> GSMTDGDYDYLIKLLALGDSGVGKTTFLYRYTDNKFNPKFITTVGIDFREKRVVYDTQGADGASGKAFKVHLQLWDTAGLERFRSLTTAFFRDAMGFLLMFDLTSQQSFLNVRNWMSQLQANAYCENPDIVLIGNKADLPDQREVNERQARELAEKYGIPYFETSAATGQ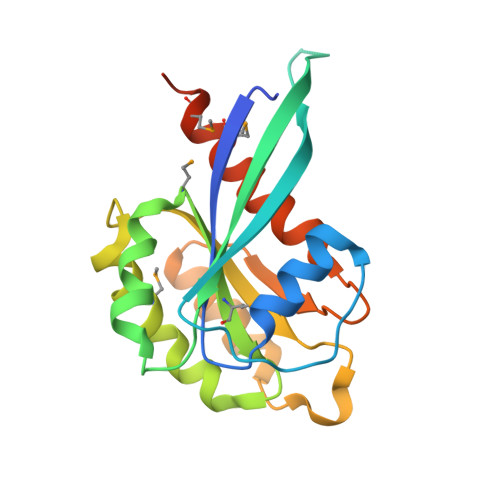NVEKSVETLLDLIMKRMEKCVEKTQVPDTVNGG> MAHHGVSGLVGKLVTQLEVNCDADIFYKIVKHHEEVPNVIPHFFTGVQVTKGDGLVSGCIKEWNYVLEGKAMTAVEETTHADETRTLTHHITEGDAMKDYKKFDVIVETNPKPNGHGSVVTYSIVYEKINEDSPAPFDYLKFFHQNIVDMSAHISSSA

Several proteins from plant pathogenesis-related family 10 (PR10) are highly abundant in the latex of opium poppy and have recently been shown to play diverse and important roles in the biosynthesis of benzylisoquinoline alkaloids (BIAs). PR10-10 has been proposed to act as a noncatalytic BIA binding protein. We observed that an intermolecular disulfide bond between Cys59 and Cys155 is formed in the apo structure, while the binding of alkaloid compounds to the central hydrophobic pocket induces conformational changes that prevent the formation of this intermolecular disulfide bond.

To decouple ligand binding from disulfide-bond formation, each of the two highly conserved cysteine residues (Cys59 and Cys155) in PR10-10 was replaced with serine using site-directed mutagenesis. A crystal structure of the Cys155Ser mutant was also determined in the absence of exogenous BIA compounds. Attempts to crystallize the Cys59Ser and Cys155Ser mutants of PR10-10 in the absence of BIA ligands surprisingly yielded crystals with the morphology characteristic of PR10-10 with bound BIA ligands. Data processing confirms that these crystals show C2221 space-group symmetry, and structure determination and refinement reveal a closed cap-loop conformation similar to the structures of PR10-10 with bound BIA ligands. Despite the absence of exogenously added ligands during crystallization, there appears to be electron density in the hydrophobic pocket corresponding to an unidentified compound. Mutation of either Cys59 or Cys155 was associated with the binding of an unknown molecule in the absence of an alkaloid ligand, whereas similar conditions for the purification, storage and crystallization of wild-type PR10-10 resulted in the apo conformation. Although holo PR10-10 and cysteine-mutant PR10-10 structures all showed closed cap-loop conformations, and slight differences in the cap position from residues 37–40 were observed, it should be noted that residues 34–36 in wild-type PR10-10, residues 35–36 in PR10-10-Cys155Ser and residues 34–36 in PR10-10-Cys59Ser–papaverine were not sufficiently well ordered to be modeled. The PR10-10-Cys59Ser and PR10-10-Cys155Ser structures demonstrated a similar cap-loop conformation, which was fully modeled for PR10-10-Cys59Ser. Residues 38–40 were shifted ∼3.8 Å perpendicularly away from the central α2 helix in the PR10-10 cysteine mutants compared with wild-type holo PR10-10.>MLKGIPKIIPPELLKVLCEMGHGDQLVIADGNFPAESIGKNAIVVRMDG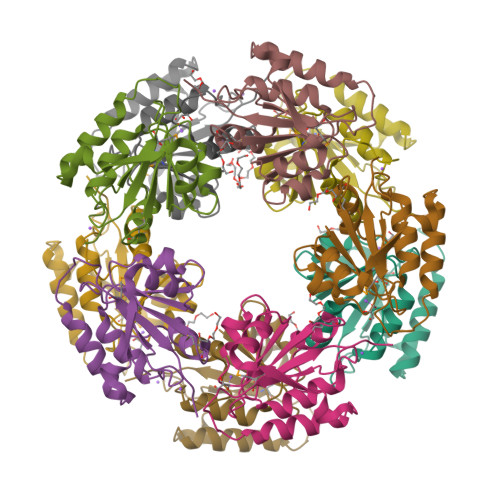HGGGEILKAILTVFPLDTYVDKPATLMEKVPGDTVATPIWDVYAGLIKEHDERGADAIGSLERFAFYEQAKNAYCVIASGESAQYANLILQKGVVFNAE[10x]> ADPLVPHLGDREKRDSVCPQGKYIHPQNNSICCTKCHKGTYLYNDCPGPGQDTDCRECESGSFTASENHLRHCLSCSKCRKEMGQVEISSCTVDRDTVCGCRKNQYRHYWSENLFQCFNCSLCLNGTVHLSCQEKQNTVCTCHAGFFLRENECVSCSNCKKSLECTKLCL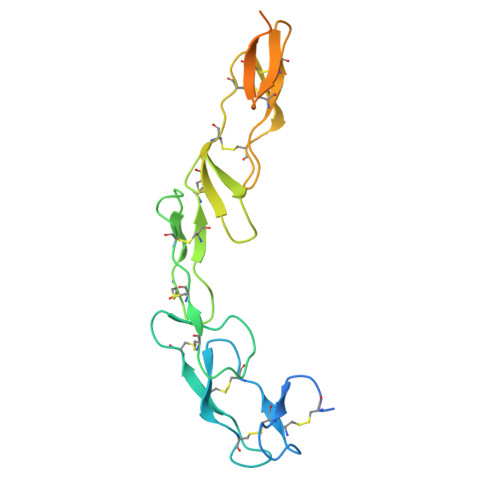PQIENVKGTEDSGTTGGGGSHHHHHHHH> SGPLGSEAHLYMQVQIVAEDQFCGHQGNDMYDEEKVKYTVFKVLKNSSLAEFVQSLSQTMGFPQDQIRLWPMQARSNGTKRPAMLDNEADGNKTMIELSDNENPWTIFLETVDPELAASGATLPKFDKDHDVMLFLKMYDPKTRSLNYCGHIYTPISCKIRDLLPVMCDRAGFIQDTSLILYEEVKPNLTERIQDYDVSLDKALDELMDGDIIVFQKDDPENDNSELPTAKEYFRDL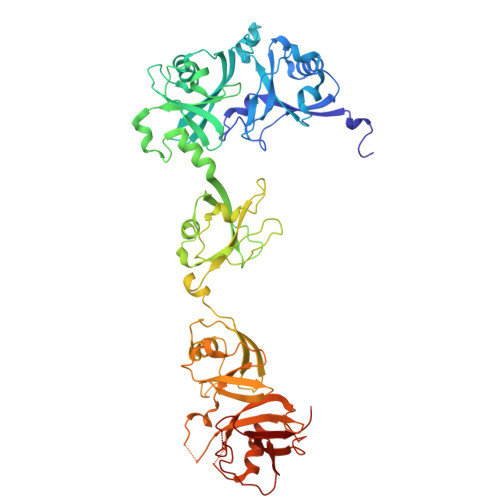YHRVDVIFCDKTIPNDPGFVVTLSNRMNYFQVAKTVAQRLNTDPMLLQFFKSQGYRDGPGNPLRHNYEGTLRDLLQFFKPRQPKKLYYQQLKMKITDFENRRSFKCIWLNSQFREEEITLYPDKHGCVRDLLEECKKAVELGEKASGKLRLLEIVSYKIIGVHQEDELLECLSPATSRTFRIEEIPLDQVDIDKENEMLVTVAHFHKEVFGTFGIPFLLRIHQGEHFREVMKRIQSLLDIQEKEFEKFKFAIVMMGRHQYINEDEYEVNLKDFEPQPGNMSHPRPWLGLDHFN>[2x]PEAPYASLTEIEHLVQSVCKSYRETCQLRLEDLLRQRSNIFSREEVTGYQRKSMWEMWERCAHHLTEAIQYVVEFAKRLSGFMELCQNDQIVLLKAGAMEVVLVRMCRAYNADNRTVFFEGKYGGMELFRALGCSELISSIFDFSHSLSALHFSEDEIALYTALVLINAHRPGLQEKRKVEQLQYNLELAFHHHLCKTHRQSILAKLPPKGKLRSLC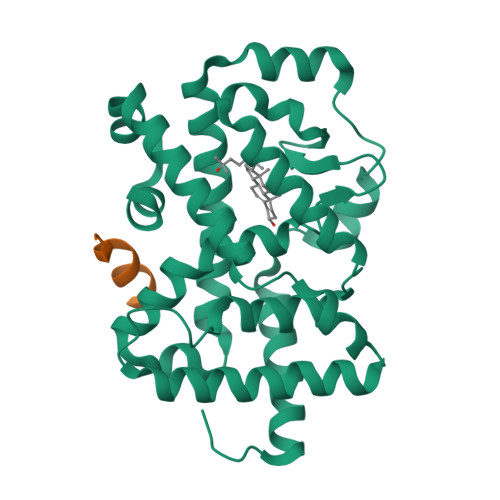SQHVERLQIFQHLHPIVVQAAFPPLYKELFS;>[2x]EKHKILHRLLQDS> GGGUUAUGUGUGCCCGGCAUGGGUGCAGUCUAUAGGGUGAGAGUCCCGAACUGUGAAGGCAGAAGUAACAGUUAGCCUAACGCAAGGGUGUCCGUGGCGACAUGG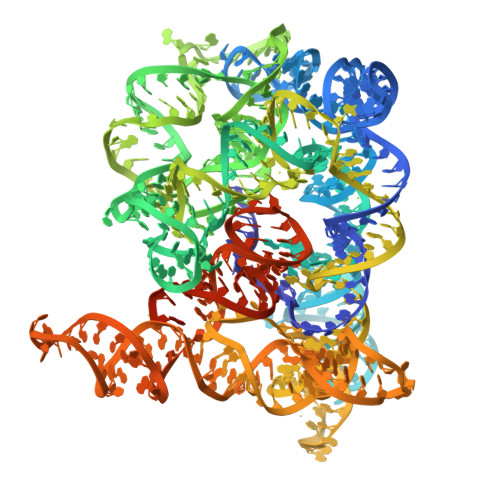AAUCUGAAGGAAGCGGACGGCAAACCUUCGGUCUGAGGAACACGAACUUCAUAUGAGGCUAGGUAUCAAUGGAUGAGUUUGCAUAACAAAACAAAGUCCUUUCUGCCAAAGUUGGUACAGAGUAAAUGAAGCAGAUUGAUGAAGGGAAAGACUGCAUUCUUACCCGGGGAGGUCUGGAAACAGAAGUCAGCAGAAGUCAUAGUACCCUGUUCGCAGGGGAAGGACGGAACAAGUAUGGCGUUCGCGCCUAAGCUUGAACCACCGUAUACCGAACGGUACGUACGGUGGUGUGAGAGGAGUUCGCUCUACUCUAUUAG> QQTIQTTLLIIGGGPGGYVAAIRAGQLGIPTVLVEGQALGGTCLNIGCIPSKALIHVAEQFHQASRFTEPSPLGISVASPRLDIGQSVAWKDGIVDRLTTGVAALLKKHGVKVVHGWAKVLDGKQVEVDGQRIQCEHLLLATGSSSVELPMLPLGGPVISSTEALA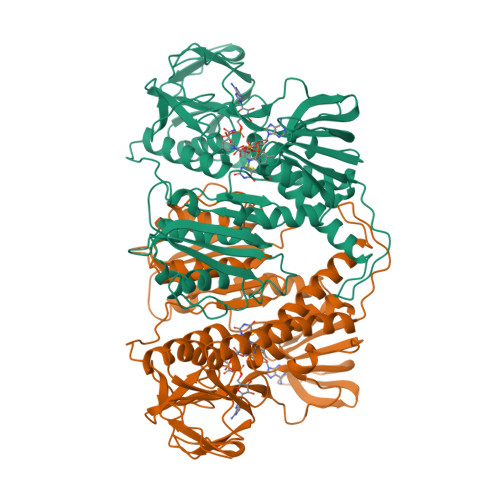PKALPQHLVVVGGGYIGLELGIAYRKLGAQVSVVEARERILPTYDSELTAPVAESLKKLGIALHLGHSVEGYENGCLLANDGKGGQLRLEADRVLVAVGRRPRTKGFNLECLDLKMNGAAIAIDERCQTSMHNVWAIGDVAGEPMLAHRAMAQGEMVAEIIAGKARRFEPAAIAAVCFTDPEVVVVGKTPEQASQQGLDCIVAQFPFAANGRAMSLESKSGFVRVVARRDNHLILGWQAVGVAVSELSTAFAQSLEMGACLEDVAGTIHAHPTLGEAVQEAALRALGHALHI2-methyl-5-(propan-2-yl)benzene-1,4-diol 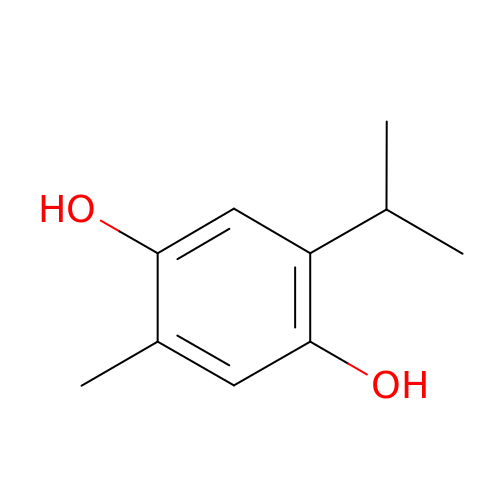| C10 H14 O2 | OQIOHYHRGZNZCW-UHFFFAOYSA-N>AKEAPQAHKAVELSILHINDHHSYLEPHETRINLNGQQTKVDIGGFSAVNAKLNKLRKKYKNPLVLHAGDAITGTLYFTLFGGSADAAVMNAGNFHYFTLGNHEFDAGNEGLLKLLEPLKIPVLSANVIPDKSSILYNKWKPYDIFTVDGEKIAIIGLDTVNKTVNSSSPGKDVKFYDEIATAQIMANALKQQGINKIILLSHAGSEKNIEIAQKVNDIDVIVTGDSHYLYGNDELRSLKLPVIYEYPLEFKNPNGEPVFVMEGWAYSAVVGDLGVKFSPEGIASITRKIPHVLMSSHKLQVKNSEGKWAELTGDERKKALDTLK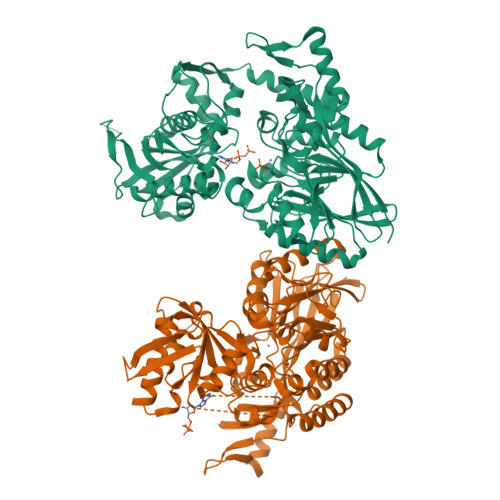SMKSISLDDHDAKTDKLIAKYKSEKDRLAQEIVGVITGSAMPGGSANRIPNKAGSNPEGSIATRFIAETMYNELKTVDLTIQNAGGVRADILPGNVTFNDAYTFLPFGNTLYTYKMEGSLVKQVLEDAMQFALVDGSTGAFPYGAGIRYEANETPNAEGKRLVSVEVLNKQTQQWEPIDDNKRYLVGTNAYVAGGKDGYKTFGKLFNDPKYEGVDTYLPDAESFIKFMKKHPHFEAYTSSNVKFNASTDALPKK[2x]> MAEDPDPTEYLYISMEQKRKDQTKPYDGKKMVWVADEKEGYLLGLIKSTQGDICTVDIEGQESRQVKKDLLQQVNPPKYEKCEDMSNLTYLNDASVLHNLKQRYYANLIYTYSGLFCVAINPYKRFPIYTNRTVQIYKGRRRTEVPPHLFAISDGAYSAMLANRENQSMLITGESGAGKTENTKKVIAYYANVGAATPKPGKEAPTKEKKATLEDQVVQTNPVLEAFGNAKTVRNDNSSRFGKFIRIHFGPMGKLAGADIETYLLEKARVISQQTLERSYHIFYQLMSGGIENLKADLLLSDDIYDYHFVSQGKIEIPGVDDAEELRLTDTAFDILGFSHEYKTDVYKITASCMHLGEMKFKQRPREEQAEADGTEEGERVAHLLGVNAADLYKNLVKPKIKVGNEMVTQGRNATQVSYSVGGLAKAMFDRTFKWLVKRLNETLDTKQKRQYFIGVLDIAGFEIFDYNGFEQLCINFTNEKLQQFFNHHMFVLEQEEYKREGIDWVFIDFGLDLAACIELIEKPMGILSILEEESMFPKATDKSFQDKLNANHLGKSPNFVKPKPPKPGQQEAHFSIAHYAGTVPYNITGWLEKNKDPVNDTVVDQFKKGSNKLVQEIFEDHPGLGAEEKGGGGKGGGGRKKGASFQTVSALYREQLNRLMASLHSTQPHFVRCIIPNELKQPGVIDSGLVMHQLTCNGVLEGIRICRKGFPNRMVYPDFKQRYTILAASAVPKGFVDAKKVTEAVLGAIQLDANDYRLGNTKVFFRAGVLGRLEEMRDDRLGKIVTWLQAWIRWYLSKKEFKKLQEQRVALLVIQRNLRKFLTLRNWLWYKLYIKVKPLLTMAKVEDELKALEEKLKKALESLEKEEKVRKDIEVQNVKLLQEKNDLFLQLESERSGAGDVEERLTKAISMKNDLEGQVQELQERLSREEDAHSNLSSVRKKLDGEISNLKKEIEDLQLVIQKTEQDKAAKDHQIRNLNDEIAHQDELINKLNREKKQMQEMGQKTGEDLQATEDKLNHMNKVKAKLEQTLDELEDSLEREKKLRGDVEKTKRKVEGDLKLAQEAVADLEKNKKELEQALQRKEKEMASLSAKLEDEQGLVAKLQKQIKELQARIEELEEELEAERQARAKAEKQRADLAREIEELSERLEEAGGATSAQVELNKRREAEMAKLRRDLEESNIQHEQTLANLRKKHNDVVAELSEQIDQLNKHKARLEKEKAQMKGELDDVRSSVDHVNKEKANAEKQAKQLEMQLTELQGKMDEAHRSLGDFDAAKKRLTVENTELTRQLEDAESQVSQLSKLKTSLQTQLEDTKRMADEESRERATAMGKFRSVEHDLDSLREQIDEEQEGKADLQRQLSKANAEVQLWRSKYESEGLARLEELEESKRKLDAKLQEAMETIDQLNSKTSGLEKTKSRLQGELEDMTIEVEKANALASAMEKKQKSFDRIISEWKQKVDDLALELDASQKECRNYSTEVFKLRSQYEESQEHYESVKRENKNLQDEIKDLVDQLGEGGRSVHELEKARKRLELEKEELQAALEEAEAALEQEENKVLRAQLELSQVRQEIDRRLQEKEEEFENTRKNHQRAIDSMQASLEAEAKGKAEALRMKKKLESDINELEIALDHSNKANAEAQKNIKKYQIQLKETQQALEEEQRARDEVREQYAMSERRCNAMHGELEESRQLLEQADRARRAADSELAELHENVNELSAQNSSLSMAKRKLEGEMQALHADLDEMLNEAKSSEEKAKKAMVDAARLADELRAEQEHAQQQEKMRKAMEGQIKELQVRLDEAEAAALKGGKKIIQKLEQKVRELETELDN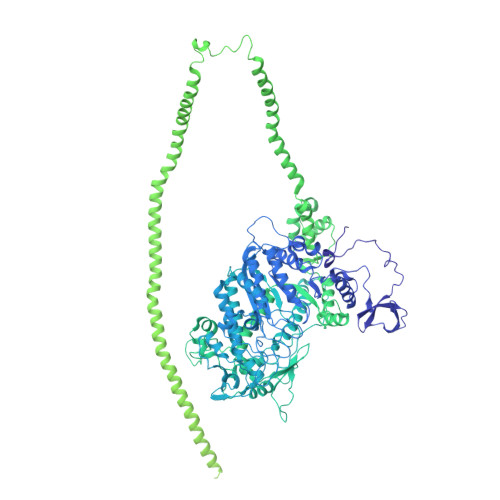EQRRHSEAAKNVRRSERRVKELQFQAEEDRKNQERMQDLVDKLQQKIKTYKRQIEEAEEIAALNLAKFRKVQQELEDAEERADMAENVAAKLRAKNRSSASVGRAMSPIPMGKPGRPKSKIDEE>MSVPAGSVSCLANALLNLRSSTDYNA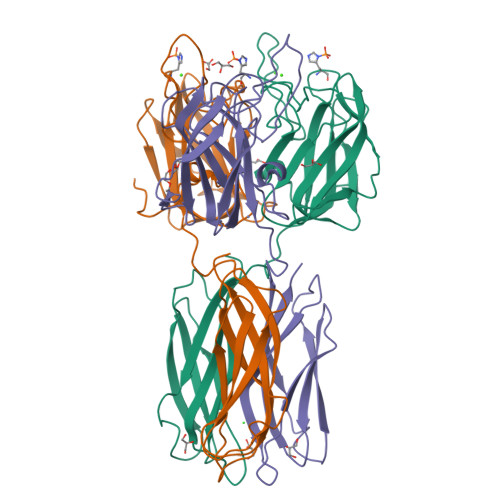DHGVKNSILNFSNSKDASRFDGSESWSSSVLDKNQFIVAGSDSVKHFVAISTQGRGDHDQWVTSYKLRYTLDNVNWVEYNNGEIINANKDRNSIVTINFNPPIKARSIAIHPQTYNNHISLRWELYALPVKSYSNPSVQVGEVSIGDRSLNSGTGSRTIVRHVKFPVEFLSVPIVSIGCKKVDAHTDNGQMRWEGKSENITTKGFDLTFITWGNNAVYDLTFDYVAVEFNN[6x]> SQGVIGIFGDYAKAHDLAVGEVSKLVKKALSNEYPQLSFRYRDSIKKTEINEALKKIDPDLGGTLFVSNSSIKPDGGIVEVKDDYGEWRVVLVAEAKHQGKDIINIRNGLLVGKRGDQDLMAAGNAIEKSHKN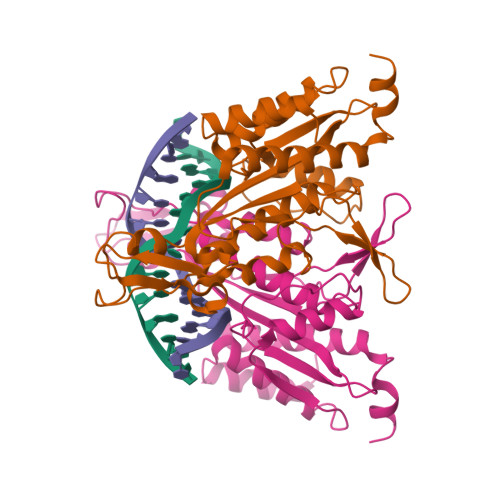ISEIANFMLSESHFPYVLFLEGSNFLTENISITRPDGRVVNLEYNSGILNRLDRLTAANYGMPINSNLCINKFVNHKDKSIMLQAASIYTQGDGREWDSKIMFEIMFDISTTSLRVLGRDLFEQLTSK>[2x]TEFLKPRLVDIEQVSSTHAKVTLEPLERGFGHTLGNALRRILLSSMPGCAVTEVEIDGVLHEYSTKEGVQEDILEILLNLKGLAVRVQGKDEVILTLNKSGIGPVTAADITHDGDVEIVKPQHVICHLTDENASISMRIKVQRGRGYVPASTRIHSEEDERPIGRLLVDACYSPVERIAYNVEAARVEQRTDLDKLVIEMETNGTIDPEEAIRRAATILAEQLEAFVDLRD;> YSYTEKKRIRKDFGKRPQVLDVPYLLSIQLDSFQKFIEQDPEGQYGLEAAFRSVFPIQSYSGNSELQYVSYRLGEPVFDVQECQIRGVTYSAPLRVKLRLVIYEREAPEGTVKDIKEQEVYMGEIPLMTDNGTFVINGTERVIVSQLHRSPGVFFDSDKGKTHSSGKVLYNARIIPYRGSWLDFEFDPKDNLFVRIDRRRKLPATIILRALNYTTEQILDLFFEKVIFEIRDNKLQMELVPERLRGETASFDIEANGKVYVEKGRRITARHIRQLEKDDVKLIEVPVEYIAGKVVAKDYIDESTGELICAANMELSLDLLAKLSQSGHKRIETLFTNDLDHGPYISETLRVDPTNDRLSALVEIYRMMRPGEPPTREAAESLFENLFFSEDRYDLSAVGRMKFNRSLLREEIEGSGILSKDDIIDVMKKLIDIRNGKGEVDDIDHLGNRRIRSVGEMAENQFRVGLVRVERAVKERLSLGDLDTLMPQDMINAKPISAAVKEFFGSSQLSQFMDQNNPLSEITHKRRISALGPGGLTRERAGFEVRDVHPTHYGRVCPIETPEGPNIGLINSLSVYAQTNEYGFLETPYRKVTDGVVTDEIHYLSAIEEGNYVIAQANSNLDEEGHFVEDLVTCRSKGESSLFSRDQVDYMDVSTQQVVSVGASLIPFLEHDDANRALMGANMQRQAVPTLRADKPLVGTGMERAVAVDSGVTAVAKRGGVVQYVDASRIVIKVN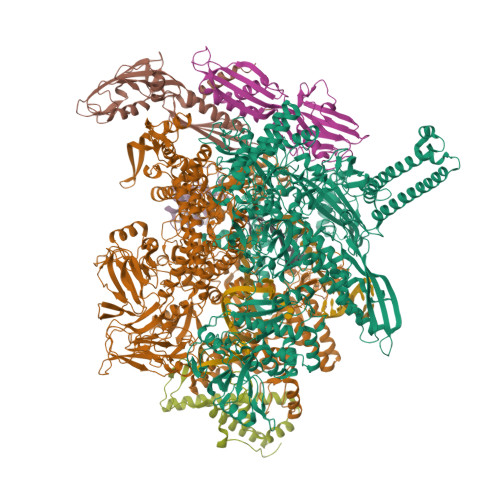EDEMYPGEAGIDIYNLTKYTRSNQNTCINQMPCVSLGEPVERGDVLADGPSTDLGELALGQNMRVAFMPWNGYNFEDSILVSERVVQEDRFTTIHIQELACVSRDTKLGPEEITADIPNVGEAALSKLDESGIVYIGAEVTGGDILVGKVTPKGETQLTPEEKLLRAIFGEKASDVKDSSLRVPNGVSGTVIDVQVFTRDGVEKDKRALEIEEMQLKQAKKDLSEELQILEAGLFSRIRAVLVAGGVEAEKLDKLPRDRWLELGLTDEEKQNQLEQLAEQYDELKHEFEKKLEAKRRKITQGDDLAPGVLKIVKVYLAVKRRIQPGDKMAGRHGNKGVISKINPIEDMPYDENGTPVDIVLNPLGVPSRMNIGQILETHLGMAAKGIGDKINAMLKQQQEVAKLREFIQRAYDLGADVRQKVDLSTFSDEEVMRLAENLRKGMPIATPVFDGAKEAEIKELLKLGDLPTSGQIRLYDGRTGEQFERPVTVGYMYMLKLNHLVDDKMHARSTGSYSLVTQQPLGGKAQFGGQRFGEMEVWALEAYGAAYTLQEMLTVKSDDVNGRTKMYKNIVDGNHQMEPGMPESFNVLLKEIRSLGINIELEDE;> TEEFDAIKIALASPDMIRSWSFGEVKKPETINYRTFKPERDGLFCARIFGPVKDYECLCGKYKRLKHRGVICEKCGVEVTQTKVRRERMGHIELASPTAHIWFLKSLPSRIGLLLDMPLRDIERVLYFESYVVIEGGMTNLERQQILTEEQYLDALEEFGDEFDAKMGAEAIQALLKSMDLEQECEQLREELNETNSETKRKKLTKRIKLLEAFVQSGNKPEWMILTVLPVLPPDLRPLVPLDGGRFATSDLNDLYRRVINRNNRLKRLLDLAAPDIIVRNEKRMLQEAVDALLDNGRRGRAITGSNKRPLKSLADMIKGKQGRFRQNLLGKRVDYSGRSVITVGPYLRLHQCGLPKKMALELFKPFIYGKLELRGLATTIKAAKKMVEREEAVVWDILDEVIREHPVLLNRAPTLHRLGIQAFEPVLIEGKAIQLHPLVCAAYNADFDGDQMAVHVPLTLEAQLEARALMMSTNNILSPANGEPIIVPSQDVVLGLYYMTRDCVNAKGEGMVLTGPKEAERLYRSGLASLHARVKVRITEYEKDANGELVAKTSLKDTTVGRAILWMIVPKGLPYSIVNQALGKKAISKMLNTCYRILGLKPTVIFADQIMYTGFAYAARSGASVGIDDMVIPEKKHEIISEAEAEVAEIQEQFQSGLVTAGERYNKVIDIWAAANDRVSKAMMDNLQTETVINRDGQEEKQVSFNSIYMMADSGARGSAAQIRQLAGMRGLMAKPDGSIIETPITANFREGLNVLQYFISTHGARKGLADTALKTANSGYLTRRLVDVAQDLVVTEDDCGTHEGIMMTPVIEGGDVKEPLRDRVLGRVTAEDVLKPGTADILVPRNTLLHEQWCDLLEENSVDAVKVRSVVSCDTDFGVCAHCYGRDLARGHIINKGEAIGVIAAQSIGEPGTQLTMRTFHIGGAASRAAAESSIQVKNKGSIKLSNVKSVVNSSGKLVITSRNTELKLIDEFGRTKESYKVPYGAVLAKGDGEQVAGGETVANWDPHTMPVITEVSGFVRFTDMIDGQTITRQTDELTGLSSLVVLDSAERTAGGKDLRPALKIVDAQGNDVLIPGTDMPAQYFLPGKAIVQLEDGVQISSGDTLARIPQESGGTKDITGGLPRVADLFEARRPKEPAILAEISGIVSFGKETKGKRRLVITPVDGSDPYEEMIPKWRQLNVFEGERVERGDVISDGPEAPHDILRLRGVHAVTRYIVNEVQDVYRLQGVKINDKHIEVIVRQMLRKATIVNAGSSDFLEGEQVEYSRVKIANRELEANGKVGATYSRDLLGITKASLATESFISAASFQETTRVLTEAAVAGKRDELRGLKENVIVGRLIPAGTGYAYHQDRMRRRAAG;> ARVTVQDAVEKIGNRFDLVLVAARRARQMQVGGKDPLVPEENDKTTVIALREIEEGLINNQILDVRERQEQQEQEA;> MTKITVNYTVDVKDIQPKHVRSESNPQNQNKIRRAWVLSLSDNAMEVIQNKIKSAPARHAYYEAIDREVSNKWIELMRKHTTESLNAGAKFIMTSCGERLEDDYCGNADERLIVAAQIVAETIAADFNR> SMQGP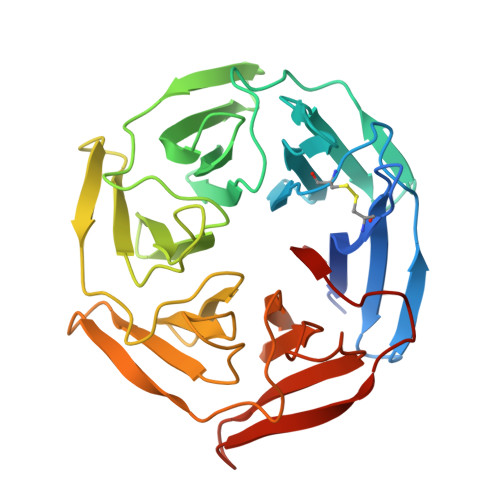RTRPRKPIRCGEVLFAVGGWCSGDAISSVERYDPQTNEWRMVASMSKRRCGVGVSVLDDLLYAVGGHDGSSYLNSVERYDPKTNQWSSDVAPTSTCRTSVGVAVLGGFLYAVGGQDGVSCLNIVERYDPKENKWTRVASMSTRRLGVAVAVLGGFLYAVGGSDGTSPLNTVERYNPQENRWHTIAPMGTRRKHLGCAVYQDMIYAVGGRDDTTELSSAERYNPRTNQWSPVVAMTSRRSGVGLAVVNGQLMAVGGFDGTTYLKTIEVFDPDANTWRLYGGMNYRRLGGGVGVIK>[4x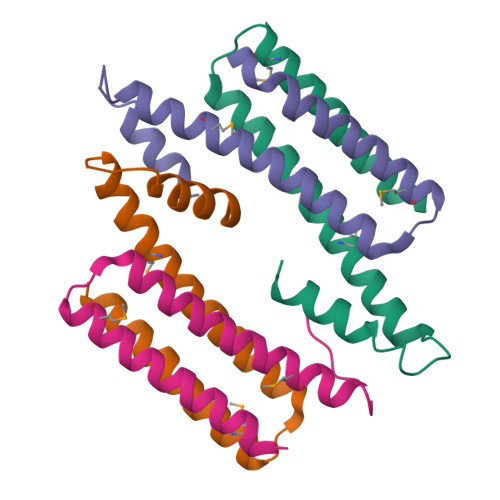]GTNSKYITALKRSEGQLRGIQKMIEGDRDCADIVTQLTAVRSSVERVIEMIITENLTECINQPLDDSEAQKERLEKAIRYLIKRK>[2x]VIHVTKEVKEVATLSCGHNVSVEELAQTRIYWQKEKKMVLTMMSGDMNIWPEYKNRTIFDITNNLSIVILALRPSDEGTYECVVLKYEKDAFKREHLAEVTLSVKADFPTPSISDFEIPTSNIRRIICSTSGGFPEPHLSWLENGEELNAINTTVSQDPETELYAV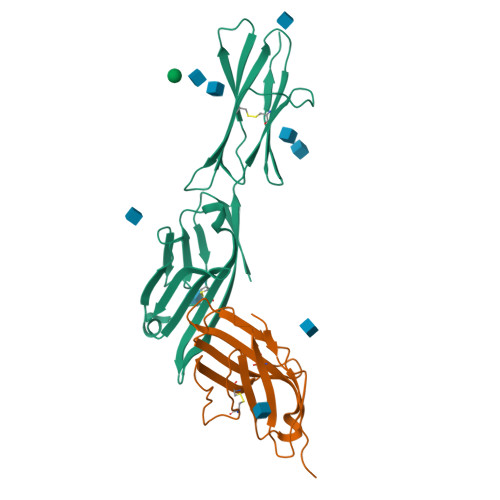SSKLDFNMTTNHSFMCLIKYGHLRVNQTFNWNTTKQEHFPDN;>[2x]KAMHVAQPAVVLASSRGIASFVCEYASPGKATEVRVTVLRQADSQVTEVCAATYMMGNELTFLDDSICTGTSSGNQVNLTIQGLRAMDTGLYICKVELMYPPPYYLGIGNGAQIYVIDPEPCPDSD> LKESPSGYLRSGEGDTGCGELVWVGEPLTLRTAETITGKYGVWMRDPKPTYPYTQETTWRIDTVGTDVRQVFEYDLISQFMQGYPSKVHILPRPLESTGAVVYSGSLYFQGAESRTVIRYELNTETVKAEKEIPGAGYHGQFPYSWGGYTDIDLAVDEAGLWVIYSTDEAKGAIVLSK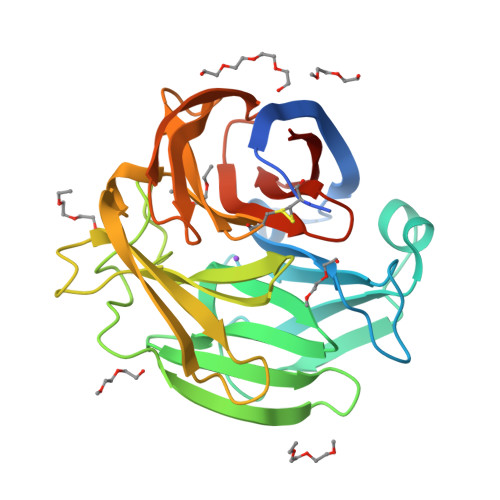LNPENLELEQTWETNIRKQSVANAFIICGTLYTVSSYTSADATVNFAYDTGTGISKTLTIPFKNRYKYSSMIDYNPLEKKLFAWDNLNMVTYDIKLSKM> MSRNTEATDDVKTWTGGPLNYKEGFFTQLATDELAKGINEEVVRAISAKRNEPEWMLEFRLNAYRAWLEMEEPHWLKAHYDKLNYQDYSYYSAPSCGNCDDTCASEPGAVQQTGANAFLSKEVEAAFEQLGVPVREGKEVAVDAIFDSVSVATTYREKLAEQGIIFCSFGEAIHDHPELVRKYLGTVVPGNDNFFAALNAAVASDGTFIYVPKGVRCPMELSTYFRINAEKTGQFERTILVADEDSYVSYIEGCSAPVRDSYQLHAAVVEVIIHKNAEVKYSTVQNWFPGDNNTGGILNFVTKRALCEGENSKMSWTQSETGSAITWKYPSCILRGDNSIGEFYSVALTSGHQQADTGTKMIHIGKNTKSTIISKGISAGHSQNSYR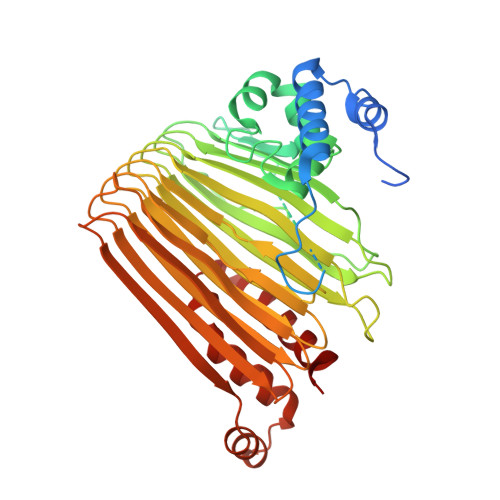GLVKIMPTATNARNFTQCDSMLIGANCGAHTFPYVECRNNSAQLEHEATTSRIGEDQLFYCLQRGISEEDAISMIVNGFCKDVFSELPLEFAVEAQKLLAISLEHSVG> MNGDETKKVESEYIKKHHRHELVESQCSSTLVKHIKAPLHLVWSIVRRFDE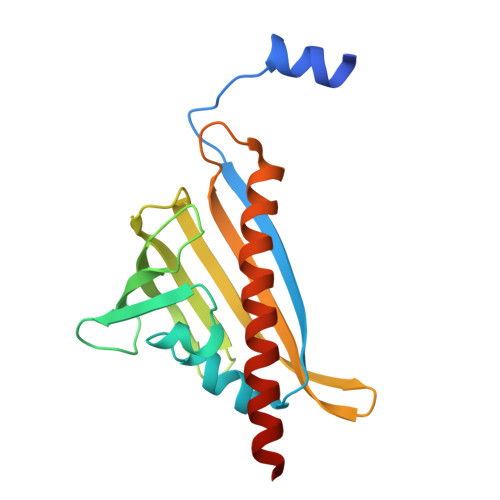PQKYKPFISRCVVQGKKLEVGSVREVDLKSGLPATKSTEVLEILDDNEHILGIRIVGGDHRLKNYSSTISLHSETIDGKTGTLAIESFVVDVPEGNTKEETCFFVEALIQSNLNSLADVTERLQAESMEKKI>[2x]SHPDLNKLLELWPHIQEYQDLALKHGINDIFQDNGGKLLQVLLITGLTV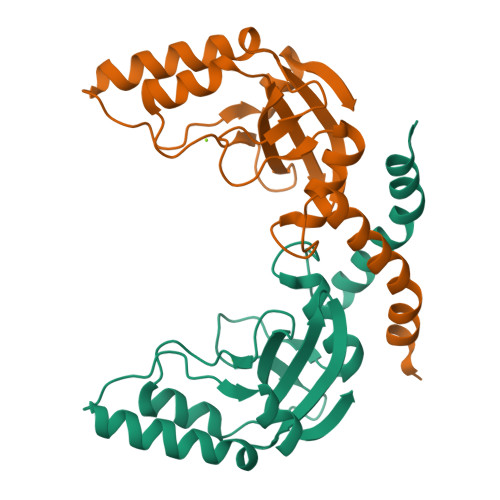LPGREGNDAVDNAGQEYELKSINIDLTKGFSTHHHMNPVIIAKYRQVPWIFAIYRGIAIEAIYRLEPKDLEFYYDKWERKWYSDGHKDINNPKIPVKYVMEHGTKIY> SEDEFYDAL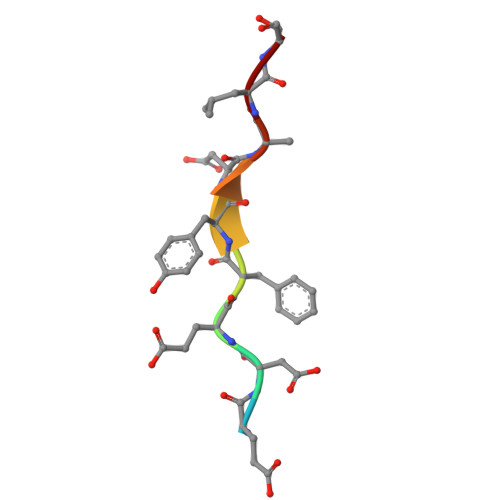S3-(3,5-dimethyl-1,2-oxazol-4-yl)-5-ethoxybenzoic acid | C14 H15 N O4 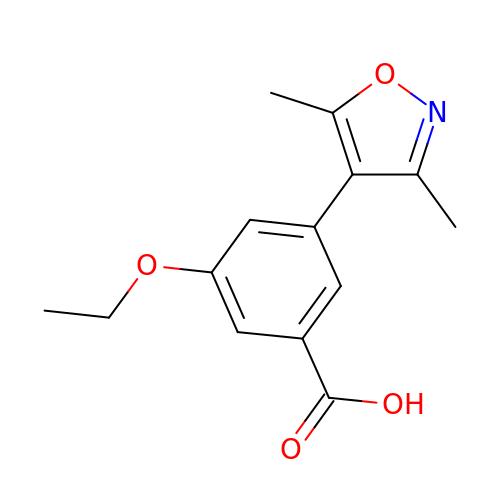| GAMMHRRBGXCHRX-UHFFFAOYSA-N The colony-stimulating factor-1 receptor (CSF1R) is a tyrosine kinase embedded in the cell membrane of macrophages. The receptor is activated by colony-stimulating factor-1 (CSF-1) and interleukin-34, and signaling via CSF1R is crucial for the differentiation, proliferation, and survival of macrophages. Unlike most kinases, CSF1R and other members of the platelet-derived growth factor receptor (PDGFR) family contain both an activation loop and a juxtamembrane domain (JM domain). In the autoinhibited form, the folding of the activation loop prevents the binding of ATP, and the JM domain forms bonding interactions with the DFG aspartate as well as other residues in the cleft between the N- and C-lobes of the protein, stabilizing an inactive form.

A protein co-crystal of CSF1R in complex with 23 was obtained using a sitting-drop vapor diffusion set-up. A complete 1.9 Å data set of the CSF1R/23 crystal was collected at the ESRF synchrotron radiation source (Grenoble, FR, beamline ID29). Inhibitor 23 binds via two hydrogen bonds to Cys-666 in the hinge backbone of the kinase: the pyrimidine N1-atom accepts a hydrogen bond from the NH of Cys-666, while the pyrrole NH donates a hydrogen bond to the Cys-666 carbonyl oxygen. Additionally, a water-mediated hydrogen bond is formed between atom N3 of the pyrimidine moiety and Thr663. The methylbenzene ring points toward the C-terminal subdomain. It is sandwiched between Leu-785 and Ala-800 and almost perpendicular to the side chain of Phe-797 from the DFG motif, which adopts the “DFG-out” conformation. Although the inhibitor binds to CSF1R in the DFG-out conformation, the ligand does not occupy the allosteric pocket that is formed underneath the αC-helix when the kinase adopts this inactive conformation, as is typically the case with type II inhibitors. Instead, the 3-methylbenzylamine moiety of compound 23 occupies a hydrophobic binding cleft formed by residues Leu-785, Ala-800, and Phe-797 termed the front pocket. The methyl group of the aromatic ring points toward the C-lobe of the kinase into a small complementary cavity in the front binding cleft. Thus, compound 23 cannot be classified as a typical type II inhibitor as its binding mode resembles that of a Type I inhibitor. The co-crystal structure of CSF1R and 23 reveals that the benzyl group of Phe-797 is folded toward the glycine residue.

> MKKGHHHHHHGQKPKYQVRWKIIESYEGNSYTFIDPTQLPYNEKWEFPRNNLQFGKTLGAGAFGKVVEATAFGLGKEDAVLKVAVKMLKSTAHADEKEALMSELKIMSHLGQHENIVNLLGACTHGGPVLVITEYCCYGDLLNFLRRKAEAMLGPSLSPGQDPEGLDKEDGRPLELRDLLHFSSQVAQGMAFLASKNCIHRDVAARNVLLTNGHVAKIGDFGLARDIMNDSNYIVKGNARLPVKWMAPESIFDCVYTVQSDVWSYGILLWEIFSLGLNPYPGILVNSKFYKLVKDGYQMAQPAFAPKNIYSIMQACWALEPTHRPTFQQICSFLQEQAQEDRR> MTESPTTHHGAAPPDSVATPVRPWSEFRLTPAEAAAAAALAARCAQRYDETDGPEFLLDAPVIAHELPRRLRTFMARARLDA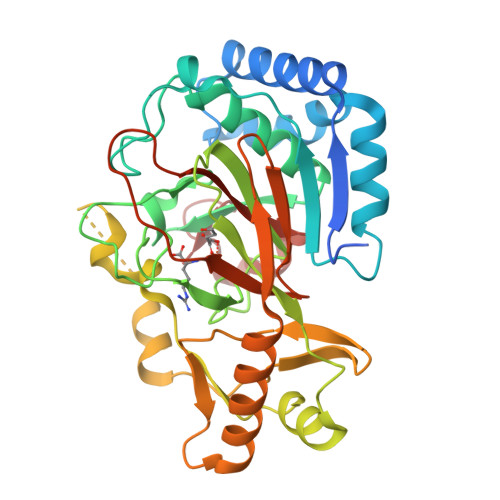WPHALVVRGNPVDDAALGSTPVHWRTARTPGSRPLSFLLMLYAGLLGDVFGWATQQDGRVVTDVLPIKGGEHTLVSSSSRQELGWHTEDAFSPYRADYVGLLSLRNPDGVATTLAGVPLDDLDERTLDVLFQERFLIRPDDSHLQVNNSTAQQGRVEFEGIAQAADRPEPVAILTGHRAAPHLRVDGDFSAPAEGDEEAAAALGTLRKLIDASLYELVLDQGDVAFIDNRRAVHGRRAFQPRYDGRDRWLKRINITRDLHRSRKAWAGDSRVLGQR>[4x]GSHMASMSEVERALDVLLQEAEELCIGSSVVELDRIPTALEFCREFYSKNQPVVIRKALNWPAIGKWTPKYLIEALGDRSVDVAITPNGYADGLATQNGQEYFVLPLETKMKLSEVVRRLDDPTGAVHYIQKQNSNLSVDLPELAADLRVSDLDFAQQSFNKPPDAVNFWLGDERAVTSMHKDPYENVYCVISGHKDFVLIPPHQLSCVPRGIYPTGVYKTSDSGQFYIEPLRDEEGSDQFTEWVSVDPLSPDLAKYPEYARAKPLKVRVHAGDILYLPNYWFHHVSQSHKCIAVNFWYDLDYDSRYCYYRMLEQMTSARSG

Jumonji domain-containing 7 (JMJD7) is a JmjC (3S)-lysyl-hydroxylase that catalyses the modification of Developmentally Regulated GTP Binding Proteins 1 and 2 (DRG1 and 2); JMJD7 has also been reported to have histone endopeptidase activity. Here we report biophysical and biochemical studies on JMJD7 from Drosophila melanogaster (dmJMJD7). Like hsJMJD7, dmJMJD7 forms a homodimer with each 316-amino-acid monomer possessing an N-terminal helix-loop-helix-fold domain (aa 1–42) that forms part of the dimerization interface, a core distorted double-stranded β-helix (DSBH, aa 160–294) fold comprising of eight parallel β-strands and an α-helical C-terminal domain (aa 296–310) which is also involved in dimerization. Notably, the crystallographic analyses on dmJMJD7 combined with previously reported crystal structures for hsJMJD720 reveal the unusual dimerization mode of JMJD7, which involves interactions between the N- and C-terminal regions of both dmJMJD7 monomers and is likely conserved in all animals making JMJD7.

We thus attempted to obtain structures of hsJMJD7 and dmJMJD7 with 2OG analogues and found that dmJMJD7 was particularly amenable to such studies. We obtained His6-dmJMJD7.Mn crystal structures in complex with the near isosteric 2OG analogue N-oxalylglycine (IC50 0.3 μM, as shown by a solid-phase extraction coupled to MS assays using DRG1 (aa 16–40) peptide substrate), N-oxalyl-D-alanine (IC50 4.14 μM), N-oxalyl-D-phenylalanine, and pyridine-2,4-dicarboxylate (2,4-PDCA, IC50 1.34 μM). The structures reveal that all four compounds bind at the dmJMJD7 2OG binding site by bidentate coordination of the metal ion trans to H175 and D177 and by interacting with the 2OG C5 carboxylate binding residues in a closely analogous bidentate manner to that observed for 2OG itself. Comparison of the dmJMJD7 crystal structures reveals a flexible region (aa 123–138) located N-terminal to the DSBH β-strands, which normally forms a loop around the dmJMJD7 active site and is likely involved in induced-fit during substrate binding. Compared to that observed in the dmJMJD7.Mn. OG/succinate/N-oxalylglycine/2,4-PDCA structures, this loop adopts a different conformation and forms a non-DSBH β-strand extending the major DSBH β-sheet in the N-oxalyl-D-alanine and N-oxalyl-D-phenylalanine complexes.>[2x]MSERTGTQPLGVQGLTEEQRMMIRELMDAQMKTFDTTFSHFKNFRLPGVLSS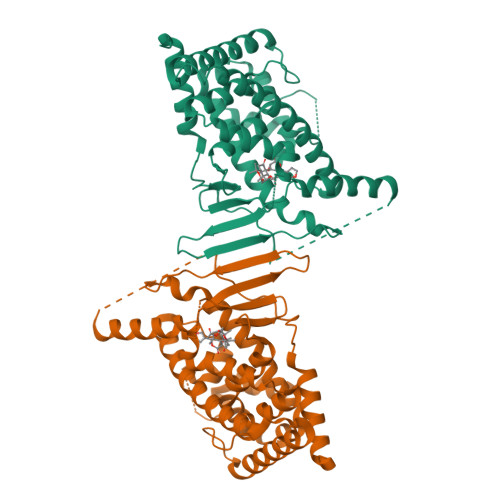GCELPESLQAPSREEAAKWSQVRKDLCSLKVSLQLRGEDGSVWNYKPPADSGGKEIFSLLPHMADMSTYMFKGIISFAKVISYFRDLPIEDQISLLKGAAFELCQLRFNTVFNAETGTWECGRLSYCLEDTAGGFQQLLLEPMLKFHYMLKKLQLHEEEYVLMQAISLFSPDRPGVLQHRVVDQLQEQFAITLKSYIECNRPQPAHRFLFLKIMAMLTELRSINAQHTQRLLRIQDIHPFATPLMQELFGITGSSSSGGTCPSSHSSLTERHKILHRLLQEGSPSAAA>[2x]MGSSHHHHHHSQDPMKIDMTEVNNQKTALANSISNLNGQIDTAKNSLTNLTSSSSLTGDVKTAIDAKINNYQVPLLTNFTNALTTLSAQYDKTIEQFQSTVSENAADAVIDTDYLQGLLDNYSGIETSISTINTETSTIYSSISD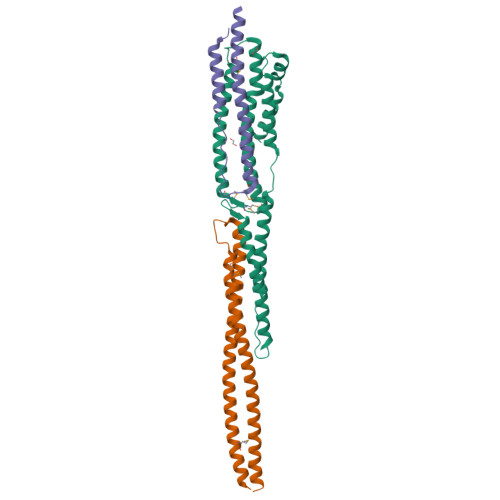IISLTNPDSSTITTPLAAAKTILTDTKTNMESFNGWTRGTELADLLLSQTQTIETLIGYASSGYTAADAKSFYNNNEFLQGVNKIAEAIANST;>[2x]MSETSASYYQDLANKESANYNNAISQKAAIDAQISRLETAKTNLSTQINNFQTDIVDKMSDIEGEDSSQFKGDRKTKYAEQYTSTKSAATTNKTSHDTNLTSITNKITELQTQSTSLQSAADTAYSNMLSYQASANAANTE;>MTKTGTDYSAWSELTSSVNTSVSGIVDLASLTFTTTTMTPFTSFNEDISSFNTAVAKLQSFTSTDVTHMNQAAENKVTDDSNQAQAQG[2x]> AGAQDFVPHTADLAELAAAAGECRGCGLYRDATQAVFGAGGRSARIMMIGEQPGDKEDLAGLPFVGPAGRLLDRALEAADIDRDALYVTNAVKHFKFTRAAGGKRRIAKTPSRTEVVACRPWLIAEMTSVEPDVVVLLGATAAKALLGNDFRVTQHRGEVLHVDDVPGDPALVATVHPSSLLRGPKEERESAFAGLVDDLRVAADVR

UdgX excises uracil from uracil-containing DNA to concurrently form a covalent bond with the resulting AP-DNA. Structurally, UdgX is highly similar to family-4 UDGs (F4-UDGs). However, UdgX is unique in possessing a flexible R-loop (105KRRIH109). Our earlier studies allowed us to propose a reaction mechanism of UdgX, which involves the formation of a covalent bond between H109 of UdgX with the C1′ position of the target deoxyribose sugar concurrently with the uracil excision from this site in DNA.

Substitutions of His109 in MsmUdgX with Ser, Gly, Ala, Gln, Cys and Lys showed the loss of its covalent complex formation with DNA but gained canonical UDG activities. However, H109 substitutions by Gln or Lys, showed poor activity. Both Cys and Ala mutations of H109 showed intermediate Kcat/Km values. Further, the overlay of all the structures of UdgX H109 mutants showed that the overall structures are very well conserved with a Cα RMSD of ca 0.2 Å. As anticipated, we note a clear difference in the sizes of the active site cavities in the various mutants. When we arranged the mutants in the order of increasing cavity sizes (left), we noted that the canonical UDG activity of the mutants increased with their increasing cavity sizes to begin with and then with a further increase in the cavity size, the UDG activity declined (right). It suggested that the initial increase in UDG activity (H109K to H109Q to H109G) occurred because of the efficiency with which the water molecule could be localized to make a nucleophilic attack on the C1′ position. However, a further increase in the cavity size (H109S to H109C to H109A) perhaps destabilizes the bound water, thereby decreasing the UDG activity.> GSSLSPTEGKGSGLQGHIIENPQYFSD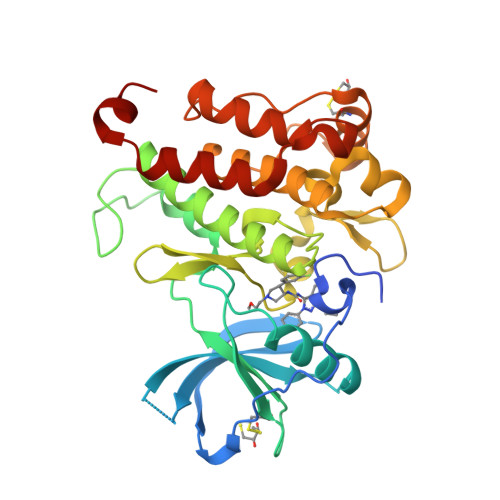ACVHHIKRRDIVLKWELGEGAFGKVFLAECHNLLPEQDKMLVAVKALKEASESARQDFQREAELLTMLQHQHIVRFFGVCTEGRPLLMVFEYMRHGDLNRFLRSHGPDAKLLAGGEDVAPGPLGLGQLLAVASQVAAGMVYLAGLHFVHRDLATRNCLVGQGLVVKIGDFGMSRDIYSTDYYRVGGRTMLPIRWMPPESILYRKFTTESDVWSFGVVLWEIFTYGKQPWYQLSNTEAIDCITQGRELERPRACPPEVYAIMRGCWQREPQQRHSIKDVHARLQALAQAPPVYLDVLG>MRGSHHHHHHGSVIFDKRIKDEEDVEKELGLPVLGSIQKFNMTNTRRSTSSLIVHEQPKSPISEKFRGIRSNIMFANPDSAVQSIVITSEAPGAGKSTIAANLAVAYAQAGYKTLIVDGDMRKPTQHYIFNLPNNEGLSSLLLNWSTYQDSIISTEIEDLDVLTSGPIPPNPSELITSRAFANLYDTLLMNYNFVIIDTPPVNTVTDAQLFSKFTGNVVYVVNSENNNKDEVKKGKELIEATGAKLLGVVLNRMPKDKSASYYAYYGTDES[2x]

We describe here the first crystal structure of a bacterial tyrosine kinase, namely CapB from the pathogen Staphylococcus aureus, in complex with the cytoplasmic domain of the transmembrane stimulatory protein CapA. CapA and CapB, among others, are involved as copolymerases in the synthesis of extracellular polysaccharides that are thought to be potent virulence factors. Reproducing the Gram-negative organization of BY-kinases by direct linkage of the Cap5A1Ct fragment (herein called CapACt) to the N-terminal extremity of Cap5B2 (herein called CapB) allowed the production of a fully active soluble protein called CapAB. The CapB kinase core possesses a P-loop type α/β mononucleotide binding fold.

The structure of the S. aureus CapAB chimeric protein was determined at 1.8 Å resolution. The refined structure of the CapAB chimeric protein includes a continuous polypeptide corresponding to residues 197a to 222a of Cap5A1 linked to residues 1b to 215b of Cap5B2. The asymmetric unit contains two molecules with a small contact surface area of about 600 Å2, characteristic of packing interactions. The crystal form of the truncated cytoplasmic domain of CapAB is thus a monomer, as observed in solution by size-exclusion chromatography (unpublished data). The CapACt fragment (residues 194a–222a) provides an additional strand called βA (residues 214a–219a) interacting with strand β7 of CapB and thus completing the central β-sheet of the protein. CapACt also contains an additional α-helix called αA (residues 202a–211a) interacting with helix α10 (residues 187b–200b) of CapB. The total surface contact area between CapACt and CapB covers about 3,000 Å2 and is highly hydrophobic, explaining why CapB is poorly soluble in the absence of CapACt (unpublished data). The active site of the protein contains ADP-Mg, most probably resulting from the hydrolysis of the 10 mM ATP-Mg contained in the crystallization solution. The adenine ring is also involved in a classical hydrophobic sandwich interaction with the side chains of CapB R212b and CapA F221a. Thus, the crystallized protein was heterogeneously phosphorylated, and the absence of electron density corresponding to the C-terminal extremity suggests that the phosphorylated tyrosine cluster is highly flexible.> LNPEQVAKIGAAIDAGRKYLDAKIEEAKKTLTLRTAQALLVIRSQYERAVDTLFTDPSAAEKELAATLATIDRLLKEHPELAAEIKAFIRSTMAEIRALLAASLAA;> LPAQVAFTPYAPEPGSTCRLREYYDQTAQMCCSKCSPGQHAKVFCTKTSDT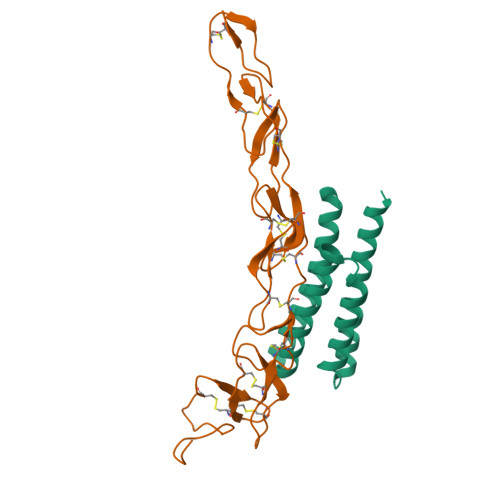VCDSCEDSTYTQLWNWVPECLSCGSRCSSDQVETQACTREQNRICTCRPGWYCALSKQEGCRLCAPLRKCRPGFGVARPGTETSDVVCKPCAPGTFSNTTSSTDICRPHQICNVVAIPGNASMDAVCTSTSPTRSMAPG>MQALRRGAAIPSRLLPRRDSWMSLAPFVAPNNAAAWRKLRDGAQEVQTVIERQSTPGKPQQIDWAKWESQIAHKDILNCLKTFYTNQVQILDRALGALETAKTPAPCEGAEKGWALFDAALSACAKSVEKSEELLSNGARALWVSCSNPPVWKVNTNEWLDSDQYWQAFVEKHHFYSQYQPGVVDPEAPQEVEAFKQAWHSRMGKFNDRSDTPMLYAYMNELPSWEYYDLHRSAFLEHMTYFLVRTGGDFRFFPEMPPWQWLAHMENLRFKLLSVAQSRRSQLQLANLERERALDFLPVDVEHHGEEYTQKFLQYETELFQACAARLMGHFMFLCDPFIPVQSAEALSAVTRVDNGKGKLFSLGDDVNALFYLPEQQRRDVERPTQAVQTLLGHLEATGRPFNPCYSELLHVHAEVLEERGEHWLTAPGECVSQAFLRRLRTDDPAYEVYCSYFKEMYERFAGAKEVSMEDGRKRLATIEKNAQEEAAAYGLALKTMGSAELAHKAREGAAKLEQLRKAQEKAAGKSAQTVQENKM[2x];>MTIHSCLARRAVSVAASGARAFASGLGARAVAVGALQSARLLHTSSLRAAGAKISPSEMSRLLEERIAGWKTQTSTEEVGRVVSVGDGIARLFGLEGVQAGELVEFQNGMTGMALNLETDNVGVVIFGDDRSVLEGDSVKRTGRIVDVPIGPGLLGRVVDALGNPIDGKGPIPAKERRRVELKAPGIIPRKSVHEPMMTGLKCVDALVPVGRGQRELIIGDRQTGKTAVAVDAIINQKEINDSTDDESKKLYCIYVAVGQKRSTVAQIVKALEQRDAMKYTTVVAATASEAAPLQFLAPYSGCAMGEWFRDSGRHCVIIYDDLSKQATAYRQMSLLLRRPPGREAYPGDVFYLHSRLLERAAKMGDKSGGGSLTALPVIETQAGDVSAYIPTNVISITDGQIFLETELFYKGIRPAINVGLSVSRVGSAAQVKAMKQVAGTMKLELAQYREVAAFAQFGSDLDASTRQLLTRGTALTELLKQRQYSPMKNSVQVCVLYCGVKGYLDPLDPKEISRFESLFIDYINANHQDILKTIETEKELSEKTEAKLRAAVDEFVAMNEFKKK[6x];>[2x]MNFSSSARWLAVRQSQTLGHTTRATVAAGRRVLAHSPAATEFTSFQSLHIGGDVCKLPLAVALGAAPSALGYGSAKHNQQRQYATLGSGWSFSKVQYTKYRITKPWTTDTTFDDIILSQPSKEDFAKFTKEAPLFLRFLKLVTDVEGRQEAFIQFAKRCENGLTVEKDVYVTKKELVDCLWKNGYTDTEINAFEIAFPADYKFHYPELAVLFDLTEEDCYKYCIRQRAATPEELVELKYTKPKNLVSSYGLCFLGVWFGLSNTVLSNAWFYSKTFPFGAVFYMLGSYFYRDIREKLWKEEKSLIHTAQENKNMGEESVYKQMKKYATDTKCLDYLSTFRTEVEDQIANYKVALVSQMRRQLTERLVEKLNGIQQAEKLIQGSLQDVMIREIVSSFKDLYKSRPELHDAAMQSAIQGLSGSDGAMDPVGAHFKASLQELAKVNLSTATADPMGTVVQRVAAVFQKREKEFLDTFTVKATEAQEIKTIVDKCHKGNTFDFHALSDEELRRLEQLYSTVNNRVGFETIHENSIKPVAPLSENSKGFVEFVNTQLEITKAKLRNARLTAFAHAFV;>[6x]MASPALQTCWRNLARLSGAQVRPSHFGAFSLGSRMSPFSSLLGARASPIATGRAGLRFLSSAAPNPGKKPASAAPPAGTNHGRITQVIGAVVDVHFDEQLPPILNSLEVQGHTNRLVLEVAQHLGENTVRTIAMDATEGLVRGQKVVDTGAPIQVPVGVETLGRIMNVIGEPVDECGPVPAKKTYSIHRAAPLFADQSTEPGLLQTGIKVVDLLAPYAKGGKIGLFGGAGVGKTVLIMELINNVANKHGGFSVFAGVGERTREGNDLYHEMMTTGVIKRKKLEDGKFDFTGSKAALVYGQMNEPPGARARVALTALSVAEYFRDEQGQDVLLFIDNIYRFTQAGSEVSALLGRIPSAVGYQPTLATDLGQLQERITTTKKGSITSVQAVYVPADDLTDPAPATTFAHLDATTVLSRQIAELGIYPAVDPLDSTSRMLAPEIVGQEHYDTARATQKLLQDYKSLQDIIAILGMDELSEEDKLVVSRARKIQRFLSQPFTVAEVFTGKPGRFVELPETIKSAQTILRGECDDLPEMAFYMCGGLEEVRSKAVKMAQEAASGK;>MGGGGGGALNKLFPGYKDKIWMKVPVQWRQQMIQHWNKSYEKQVYSESVALNRTFQARNQLVLDRLKPSGAYRLPAVDYKRQLSRGTLVEGADFYLPTAQEQQRLARHFEPYSEQEQEERRKFRFQSISVYLAVALGASFVHDYFYQRRPVAWCLEKEPPHPPSYPFWFKSLFHSHDIPSVRRGYEVYRKVCATCHSMEQLHFRHLVGEVLPEKRVKQIAAEYDVTDGPNDQGEMYTRPGILGDAFPSPYPNEEAARYANGGAYPPDLSLITAARHFGPDYLMALLGGYRDPPEGVELRPGLYWNVWFPGNAIAMPPPLMDEMIDYEDGTPCNISQMSKDVVNFLTWATEPTADERKLYGLKCVSAIAIGTVLMTLWWRFYWAMYATRRIDFGKLKYL[2x];>MSPVGRLFLGSKLPAQTWQSFRLQPALPQFAQKRFFSGGAAKPSWHVAREHRFGPTLPDHAYYGEHATYNYFVLFIRGMRPYLEKIFGDCASTIKNAAVAVYRPVNAFVVKHNPDLRLQFVAFASFIATHMAITKEFNDMYQRLVDITSLLELQAAQLHASEGFWDSESEQQEARLQRHAEHRNDLETTWEEALREATLARNFDVLVSYLNHGTSDGCGEHGACGHSGQNGIPPSVTWNFNAMPYGKENPDTKTFPIPDHEQPYRAFSLGFTANNLSGNWGDYIDRQDNKNALMRPARMMFTDVFIPTTK[2x];>MGEKQEEEGEEEKEGKGEGGGEGGREEEDEDGSAPVVSWLRIVEERECHEETDEAPETKIALPFSAQRSSRGFEARQVEVLVSANSAFLLSVLLASLFLSSSLPSFCPPRFLLSVLLALFKDKMAGDAPAAAAAPQQAGRTASASGVRTPGYLDLVGHSLKATSMDHGMQYSSIYWETSHRTYLPFWASLTQKFSWKIMDDQIRSFLRLPKPVTTEPFVFSSGSPYIRRYFGDADISVPVPLHAPAHFAFVPTGTVSPWEETGMETGPQGAAARGAAATAFRAVLESAWKCDIDEQIKEKLHSRAGAGAFHASGSTGGCPIPTDF[2x];>MALNRVPSRVLPFAVSGVYVHPRNACRLPAAAAVSSVPSSVSAFSSRTNFLSRSSSAVMSHPCAATARHFSFAIPPANAAALADPLPATPTPPPVFEAVSSASSGIASGTNALKNVEEVSTMERYEAAVYEESFKKPIVCLFFARFSLQSKVLLQPFLDFAASASNNATFFLIDCDRVPRAAYHARVENVPSLVVMKGDDAFRQTITDSVGVKTAGDLIQEARSALDQVLRLDQQEGGTKLQPGVSSYTHHIGVDNLNVYRKGWPVA[2x];>[2x]MQNGVFTRENADFLVKSGADSPSSQSLLLRTSPSPLSLPRRRFIFLRSASVDLSERSSLACLAPFFCLASGVCLRSAFSLPFFARRGRPCLFFIFIFFFRVSFTANFRGKRVKMAASTIPISQWPSLLYAPPSSPANPAVEALPEMQFDDLHYPRQMLLCRGAGYSLEQCNRMAQPDARVTPENPAEKLLKEEAVAAIACLSQREGGKDEQCRYYIERMYKLANKEKQPEPGTLSKASTLACKLLGIHRPEA;>[2x]MALPLLASRRLFSSFVFRGQPSTLSSNLSLVRIRGLHGGSLSPPSATLPRAVQLFSSRIAFSTAAAEDSGASQTLEGRYASALFRVAKKKNQLEKVYGDLESVRNALKDSSEFRLFVDSPAVSVQQKLDVLRQLVNRYKFDPLTGNLLTTLVENKRLPMLARVADAFDAMYRKEKGEVKCLVTSAKPLSAQQQKEIVAALQNRAGTQARLIIDYAVSPQIMGGLVVRLGEQVLDFSVATRLDRLQSQLLAPL;>MAETREGGQSGAASILGAEAFPELLSKVPLNPQMDEDKHFNKYKWGNEPIPVNRRTGSRMNSSIYDNRNHEAVRHPWSTDARTFHPNDNPEADRINTQYSNMVSDSFPEGGFSDAPRFSSNWERLLAYHHGLYSPEKFNSTTKTADEIRLAVNDFAAKVHADDPKNACKYLMIEEFKCLQSAQARIDPQGAATKCVKWFNEWRQCAWDQEKMVKGYNYIEDRRARKHKPYIGAPDLQYS[2x];>MFFSRLSLSALKAAPAREALPGLLSRQSFSSAGFSQFSSQKFFFSPSRNFSQSPLFQKHTPVHCNQRIASALVPTQQPAMTRQNPYAMQVGARYDAGVASLSAAIALMSVGGVAQGIGSLFAALVSGTARNPSIKEDLFTYTLIGMGFLEFLGIICVLMSAVLLYS[20x];>MPSSSSEDAQGGNRFECVSNSTSPRRKNATKDEAACLQPRRSAVSGPREDVLCIRTTPQPHVRRGKSGPGRRKRMRFGRERERRDKKRGEGERKRTRFPFLRLHIEGGNANSRRPLCFPSRHSLLRNHYGSLSMAFRKVSPPKAPMSVFEARSSFLDLEQCARAAGPQRWEAECQGVRQRALQAAADVMSRECGAYGDSFFQCYRHGFRLEACQGEKATMQLLRCQRMVADRLVPL[2x];>MGLSPAFAATAGCRLASPVANSSRFLSLLRLSRPRLNAAAPAAEAAKTLERNVPMKEILQPLWVVEPPNFLRQPVWKQFWEAQFANRSFFFFGNAWTSAAAFAFFIWWSRVFDPPPKERLDRYWLNSPKFRILSAFHNPGKRPGLKISLMTYEARYCYRGLDHPFTLNEMKDFLFKLREQYLVNKYEGIQFPFVFRQFNRVSTPGTLEVHTSPALQQQPHFHEEAAGHH[2x];>[2x]MAAGSRFPFCTAARLSSRGTLPRLGEATFFAGAESQRSAGAFAKTLQRPFLRAPSTQLFPVGNRLGVSSARALVANAMEPRRFFAAAASAKATHALQPTGTGSVAFTRPGQGSNAQFQTSLADKTRGLLGVGFLRPTKMASFAATFLLNFRFYFMYMARTTFQAVRPLLAFSVFGEVMKLVLATMSSGLFSFLFSFVLAFEVFYFFLQCYISYTFLTMFFTVLF;>[2x]MTALPPPPSANVAVSFTAAPAEP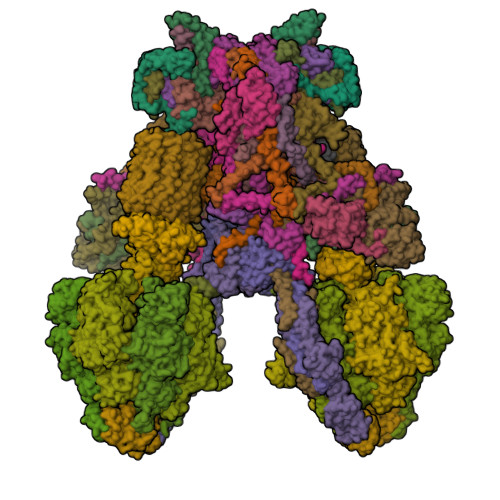LSRGEVKAASLKLELQNIERELKDWWMSRKILRDRNIGLFNLLQHHNFAGLSVNNAKLSDSQRVMWTDLVQGKPDVEDKLSVDAREMKVDMYEKLFKQAADLENPCRMPGVAYLRCLRDTLTETQSARRSSCLNAFSSFDACRTGLLKQQSAAVENSLVRQNMADVRAKALFERRAVLLDLVEGK;>[2x]MNTFFLTPAAAAARRVAVSFFARSSASGFPQHRVALRPFPSQRPAERAHNLAKSQTLRSVKAHGRQSGKKEQSTESGGRRGFRAAVGAGTGCMLAASPMLFTDYDNTASPKSELIFMAGNALGYCTERFFENEYGQSIFMFALGLAYLAMLGHEGKIHGAVWRMKHLFATNFKMVGHPRYAYALPKNPLLQDAAPTKTGSTSAKK;>MSGDSVAPHQRAACEQLHSEYKQCLAKNGRTHFSACTDFHSKLRACENMLGTSYCIDEGINLMKCTKNPDPSFCAKEFVAMRECNRPQGPHLVLSSSPSSPPHYELRPEVKHLYNVDSTDLGSAVAPVRSKEQLDRVADSLKADLNLPGYGHIPYKWESLRPNPGA[2x];>MAFAGAAAPLGVKGRSVFAGMRSFIGQRLGRLYDSFYYSQSSTKYVMVFLFPAGIFYTRFRADTKLGYHVFINEEKLYPDYSQNYFDTKWTNGRKVYLDDETTVEQLKAQIYGGKAAPENVKVACRGRVFEDADNVAMAVRAFCKRDPRLLLFQDNL[2x];>[2x]MSPPTASASVASSGSSPHMDRLLGDLKLLAAYDSAAGWQEPKAMESAFQSLSWDDADVLKALPQYLNCRGEQKRRVDFAYAALCPRPVDEKDPKQTLMSLWMKARLFSYDQKHPFVLSPFAATDKSTSAGAMTAEKPF;>[2x]MVRNQRYPASPVQEIFLPEPVPFVQFDQTAPSPNSPPAPLPSPSLSQCEEQKDRYRDISSMFHRGVAGAEQVREAYNSMAKCFRRVSVAEVLESDPAFRQARNFTMDLKQAEDDQRYKQLQYGRVPSILTKYHL;>[2x]MLNFIPKRCPSVSLLFGKRPVQRIEVGQARHQLEIPVETIEKIYEGVDSRLEYHNKDYNAMKWKDFMKLKLDAYHLLEASQSETAAKSALSDLNWFSDLADIYSGQQTMAEMDVALKAQGEQKLSYPIQGKNIK;>MSWATRLLRMSSPRLGLLPLGRSVKLGGAKERVSFSQFFDSEYFWTKANVGPFFLFLFTSPFWYQGIKTVYASCRYRKLNEREIISDRYTWLHERMLEDEVERVLLEQVPAGGFDKTRPGLLLGPSTL[2x];>MPAPAASGAAAVLSKDIARSFRWMQAFAAVKGKPTAGSCAAGTAVVNPEDPTKVTLKGRYTNFSLQHIWEKYDYLQTHLLLRECMLSQVAKNPRLLDPEINAGLTPTVFMRVPPETQDPETQAKAAPQKGQAN[2x];>MATPPLQDGAPTNGGAATKPSCGARLQNFARMAIKGPSVPHSILFGVGAGCCAYAGYYLYRAMRLTFFDTESVALQSRLRYAEKQKLFHQELDRELAAGHIASLVAEYDPVATRLPFQPMQDRYRV[2x];>MGFHFQQYIAMAGRAINPVQWTRAWRRMEGKSATEVYRDALAWTNNQFAQISRASQYRAWWWQNPLGMGLVLYGTYKAWHMIYMVRKQKKTAQLVAAAYGQGGQWLNPVPR[2x];>MPFMWRQRAYCAPVPSAFASQQPNGLGGEAGVRKPLLRSNSESLSVFSQIPDGLLGHTTSVTMGNSDIFFLPKPSNLLKIALPAFVFMPNLTIFTRAFPFYAHTSA[2x];>MSTSPGLAFANLTLLLDVPQLPAIWAVNAWRELNGLFTEMKTLAGTSDLLYPSNRYNPQNEKTNRMGRPRKYNHGEWMFGNSY[2x];>MFARAFSRFASLAAPAPQRGWNAFVLPSRHFATAAGGANPFKNQLLLTLSSPSEAIYVRTPVRSVTVPGSEGAMTMTNGHSQTVARLKAGEIIVRKGETGDEVERFFLSDGFVLFKSPEDDSGCCTAEVLGVEVVPVSMLDKESAATALQELLQQGAGATDEWTKARTLLGQELLSSVIRAAP[2x];>[2x]MWRSSGVSFTRYASEMAALLRQCLKEPYRTQAMQRNQIHLKETVYQQGQVLTRETFNDIKKAFEAAAKHAGEK;>MAGLASLSSVGALRGMRLVPAAHLLPLHSAFGQQTRNFGAGDLKIVAARMKSVKSIQKITKAMKMVAASKLRMDQRRLENGLPFATPVQKLVQRIPVDPKEKGTLAVLALSSDKGLCGGVNSFVAKQARIVIKENEMAGNAVQVYGVGDKIRSALQRTFGDRFKRIMTEVTRFPWNFGQACIIADRLMQDNPARLMVIYNHFKSAVAYDTLTLNVLTPTQAAQSAKEQLNTFEFEPEKTDVWKDLQDFYYACTVFGCMLDNIASEQSARMSAMDNASTNAGEMISSLTLRYNRARQAKITTELVEIISGANALE[2x];>MSSPCCVAIRRVARTTLESGRRQVDSKSTDVSPFFTGTQQMSLPSAGMVTKIRNFSSVKFMDQKRSGEETVYFKKEDEALLRNLLANHPEYDPKYSVDHMNAEVGSIARDITLACQKHGMKDPSAAFMKDLISIFGAHGYAKNSK[2x]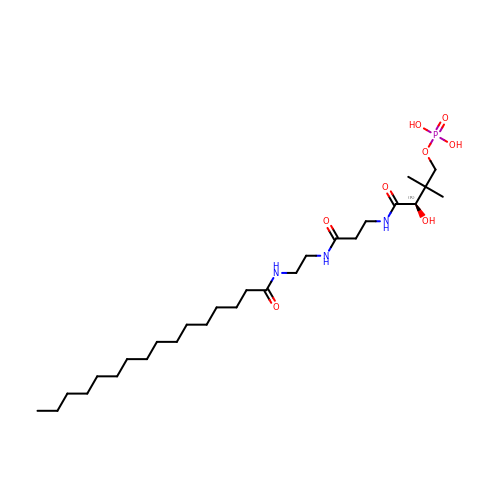N-[2-(hexadecanoylamino)ethyl]-N~3~-[(2R)-2-hydroxy-3,3-dimethyl-4-(phosphonooxy)butanoyl]-beta-alaninamide | C27 H54 N3 O8 P | KCTLTWRYJGTZMN-VWLOTQADSA-N>[2x]AEAGITGTWYAQLGDTFIVTAGADGALTGTYEAAVGNAESRYVLTGRYDSAPATDGSGTALGWTVAWKNNYRNAHSATTWSGQYVGGAEARINTQWLLTSGTTEANAWKSTLVGHDTFTKVKPSAAS;>AEAGITGTWYNQLGSTFIVTAGADGALTGTYESAVGNAESRYVLTGRYDSAPATDGSGTALGWTVAWKNNYRNAHSATTWSGQYVGGAEARINTQWLLTSGTTEANAWKSTLVGHDTFTKVKPSAASEEEEEE[2x]

The femtomolar affinity of streptavidin/avidin for biotinylated targets, combined with resilience to harsh conditions and an on-rate of ~ 107 M− 1 s− 1, is the basis for biotin's central role as a specific biological “glue” in diverse research methods and biotechnologies. We previously generated streptavidin heterotetramers with exactly one, two, or three functional biotin-binding sites, through purifying tetramers containing defined numbers of non-biotin-binding “Dead” and His6-tagged wild-type subunits. However, tetramers with two functional and two Dead subunits can assemble in three different arrangements. To generate a controlled and stable bridge for bionanotechnology, we demonstrate here a method for the simple isolation of streptavidin variants with precise cis-divalent or 1,3 trans-divalent arrangements.

However, in the 1,3 arrangement, both sites are in a trans configuration, pointing away from each other. In the first instance, we placed a hexaglutamate tag at the C-terminus of core streptavidin monomer (termed SAe). Second the C-termini are close together between subunits 1 and 3 (27 Å) but far apart between subunits 1 and 2 (57 Å) or subunits 1 and 4 (50 Å), so that elution from the ion-exchange resin would be predicted to occur later for the 1,3 divalent. SAe was refolded together with Dead (D) streptavidin (N23A, S27D, S45A). For the 1,3 trans-divalent form, crystallization with 2-methyl-2,4-pentanediol (MPD) gave us the desired asymmetric unit. The obtained 1,3 trans-divalent crystal structure was solved at 1.6 Å resolution, and cis-divalent streptavidin was solved at 1.4 Å resolution, with the phases in each case solved using molecular replacement. For the putative 1,3 trans-divalent, the electron density closely fitted residues 23, 27, and 45 only if chains b/c were SAe and chains a/d were D, confirming that the biotin-binding subunits indeed had a 1,3 trans orientation. The Dead streptavidin subunit has not been previously analyzed by crystallography, and the changes to the structure are localized to the mutated residues, consistent with the comparable thermostability of tetramers containing wild-type or Dead subunits. The overlay of D and a wild-type subunit bound to biotin illustrates how the three mutations in D greatly reduced the number of polar contacts to biotin. In the overlay, Asp27 has van der Waals clash with biotin and there would be repulsion between the Asp27 carboxylate and biotin's carbonyl oxygen lone pair.>MSGTGRLAGKIALITGGAGNIGSELTRRFLAEGATVIISGRNRAKLTALAERMQAEAGVPAKRIDLEVMDGSDPVAVRAGIEAIVARHGQIDILVNNAGSAGAQRRLAEIPLTEAELGPGAEETLHASIANLLGMGWHLMRIAAPHMPVGSAVINVSTIFSRAEYYGRIPYVTPKAALNALSQLAARELGARGIRVNTIFPGPIESDRIRTVFQRMDQLKGRPEGDTAHHFLNTMRLCRANDQGALERRFPSVGDVADAAVFLASAESAALSGETIEVTHGMELPACSETSLLARTDLRTIDASGRTTLICAGDQIEEVMALTGMLRTCGSEVIIGFRSAAALAQFEQAVNESRRLAGADFTPPIALPLDPRDPATIDAVFDWAGENTGGIHAAVILPATSHEPAPCVIEVDDERVLNFLADEITGTIVIASRLARYWQSQRLTPGARARGPRVIFLSNGADQNGNVYGRIQSAAIGQLIRVWRHEAELDYQRASAAGDHVLPPVWANQIVRFANRSLEGLEFACAWTAQLLHSQRHINEITLNIPANISATTGARSASVGWAESLIGLHLGKVALITGGSAGIGGQIGRLLALSGARVMLAARDRHKLEQMQAMIQSELAEVGYTDVEDRVHIAPGCDVSSEAQLADLVERTLSAFGTVDYLINNAGIAGVEEMVIDMPVEGWRHTLFANLISNYSLMRKLAPLMKKQGSGYILNVSSYFGGEKD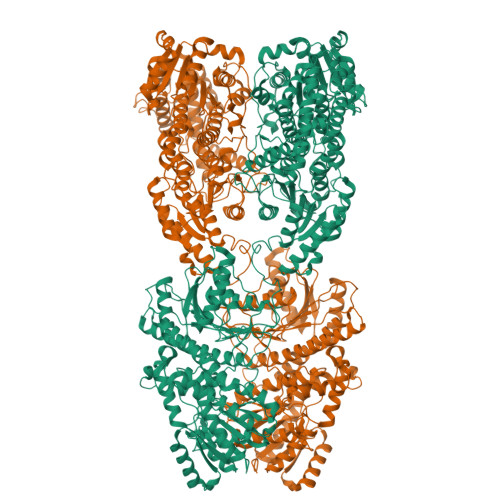AAIPYPNRADYAVSKAGQRAMAEVFARFLGPEIQINAIAPGPVEGDRLRGTGERPGLFARRARLILENKRLNELHAALIAAARTDERSMHELVELLLPNDVAALEQNPAAPTALRELARRFRSEGDPAASSSSALLNRSIAAKLLARLHNGGYVLPADIFANLPNPPDPFFTRAQIDREARKVRDGIMGMLYLQRMPTEFDVAMATVYYLADRNVSGETFHPSGGLRYERTPTGGELFGLPSPERLAELVGSTVYLIGEHLTEHLNLLARAYLERYGARQVVMIVETETGAETMRRLLHDHVEAGRLMTIVAGDQIEAAIDQAITRYGRPGPVVCTPFRPLPTVPLVGRKDSDWSTVLSEAEFAELCEHQLTHHFRVARKIALSDGASLALVTPETTATSTTEQFALANFIKTTLHAFTATIGVESERTAQRILINQVDLTRRARAEEPRDPHERQQELERFIEAVLLVTAPLPPEADTRYAGRIHRGRAITV[2x]[PROPYLAMINO-3-HYDROXY-BUTAN-1,4-DIONYL]-ISOLEUCYL-PROLINE 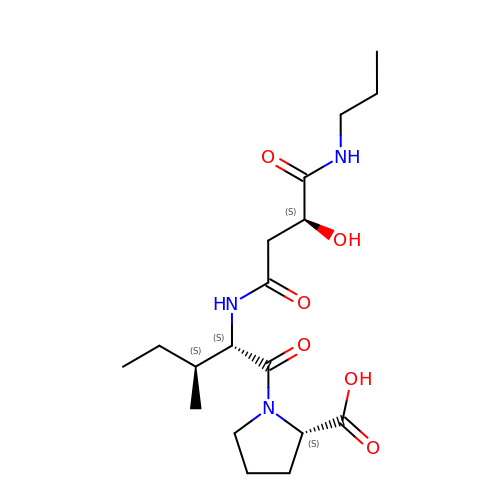| C18 H31 N3 O6 | UDNIFTKCMDIXFC-ABHRYQDASA-N>QDSTSDLIPAPPLSKVPLQQNFQDNQFHGKWYVVGFAGNAILREDKDPQKMFATIYELKEDKSYNVTSVLFRKKKCDYWIRTFVPGSQPGEFTLGNIKSYPGLTSYLVRVVSTNYNQHAMVFFKWVSQNREYFNITLYGRTKELTSELKENFIRFSKSLGLPENHIV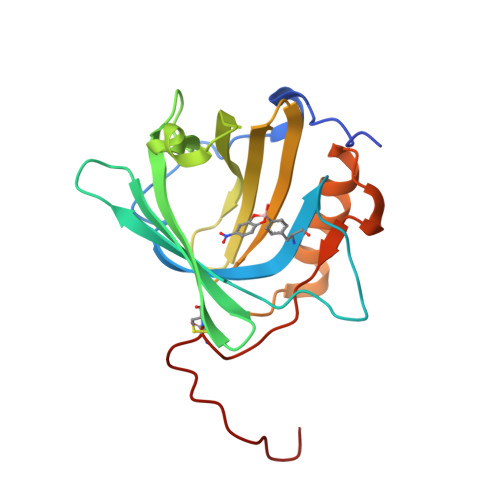FPVPIDQCIDGSAWSHPQFEK[2x]> MSLTEEFVNKEDALKNYNAKEFRTPDGYTSDMILTTVKELNGKPTLHILLIKRSL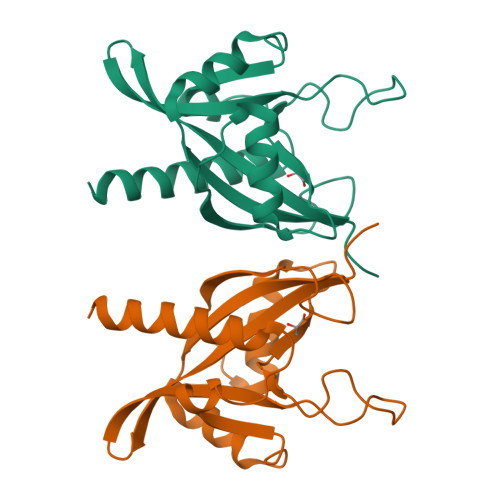TNAEGKPNMEGGKWAVPGGFVDENESAEQAAERELEEETSLTDIPLIPFGVFDKPGRDPRGWIISRAFYAIVPPEALEKRAAGDDAAEIGLFPMTEALELPLAFDHLDMLKKAFSAITEEFLLTEGHHHHHH> MGSSHHHHHHSSGLVPRGSTSEVIEDEKQFYSKAKTYWKQIPPTVDGMLGGYGHISSIDINSSRKFLQRFLREGPNKTGTSCALDCGAGIGRITKRLLLPLFREVDMVDITEDFLVQAKTYLGEEGKRVRNYFCCGLQDFTPEPDSYDVIWIQWVIGHLTD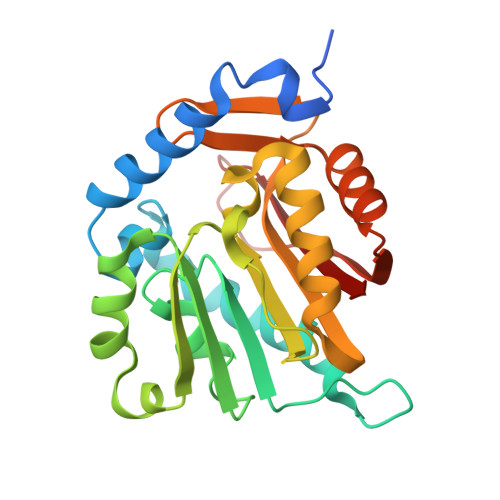QHLAEFLRRCKGSLRPNGIIVIKDNMAQEGVILDDVDSSVCRDLDVVRRIICSAGLSLLAEERQENLPDEIYHVYSFALR N-(3-oxocyclohex-1-en-1-yl)octanamide 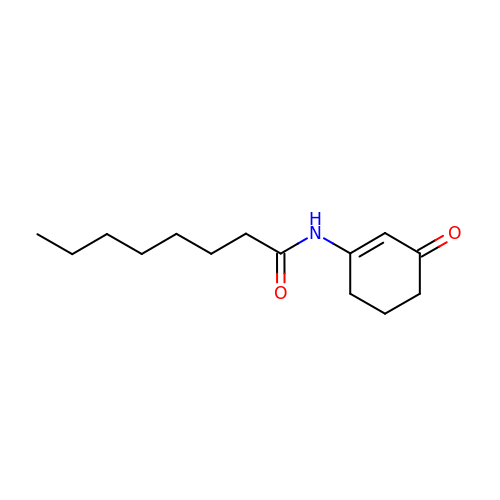| C14 H23 N O2 | USNFUKCPLYEHLS-UHFFFAOYSA-N>AMSAKDERAREILRGFKLNWMNLRDAETGKILWQGTEDLSVPGVEHEARVPKKILKCKAVSRELNFSSTEQMEKFRLEQKVYFKGQCLEEWFFEFGFVIPNSTNTWQSLIEAAPESQMMPASVLTGNVIIETKFFDDDLLVSTSRVRLFYV[4x]

RAS is a major anticancer drug target which requires membrane localization to activate downstream signal transduction. Phosphodiesterase 6δ (PDE6D) has a beta-sandwich immunoglobulin fold which contains a hydrophobic pocket capable of binding to the farnesyl group. PDE6D binds to and sequesters the lipid of cytoplasmic RAS and has been proposed to deliver GTPase to recycling endosomes, which is followed by release mediated by the small G-protein Arf-like 2 (ARL2), allowing RAS to be trafficked back to the plasma membrane. The resultant lipid modification increases the affinity of RAS proteins toward membranes, where it is required for signal transduction. Here, we present a novel strategy for targeting RAS by stabilizing its interaction with the prenyl-binding protein PDE6D and disrupting its localization.

Two cocrystal structures with the fragments identified in the screen were successfully obtained: compound-1 in a ternary complex with PDE6D and WT KRAS peptide and compound-2 in complex with PDE6D alone. In the crystal structure of the PDE6D:compound-2 complex, four copies of PDE6D are present in the asymmetric unit. This fragment, similarly to compound-1, also binds within the PDE6D cargo-binding pocket but occupies two distinct binding sites. One binding site, normally occupied by the side chain of W90, is located at the entrance of the PDE6D-binding pocket, where the fragment forms a hydrogen bond interaction with E88 and packs against W90 and V80. The second binding site is deep within the PDE6D-binding pocket, where compound-2 forms hydrophobic interactions with residues M20, L23, L38, L76, T131, and V145, as well as a weak hydrogen bond with Q78. Comparison of the PDE6D-binding pocket in PDE6D:compound-2 complex and the ternary complex containing compound-1 demonstrates that compound-2 forms limited steric clashes with the KRAS C-terminal cysteine residue when bound at the entrance of the PDE6D-binding pocket. The compound-2-binding site deep within the PDE6D cargo pocket does however overlap with the farnesyl group of KRAS and will compete with KRAS binding. Compound-1 showed no competition with KRAS in either experiment; however, compound-2 did show competition with the KRAS WT peptide. Finally, we cannot exclude the possibility that compound-2 binds at a different site or with an altered conformation when KRAS is also present within the binding pocket. Overlay of the two complexes containing compound-1 and compound-2 shows that these fragments are within close proximity to each other with a distance of 4.8 Å between the two closest atoms.>[2x]SNAMWKRMTA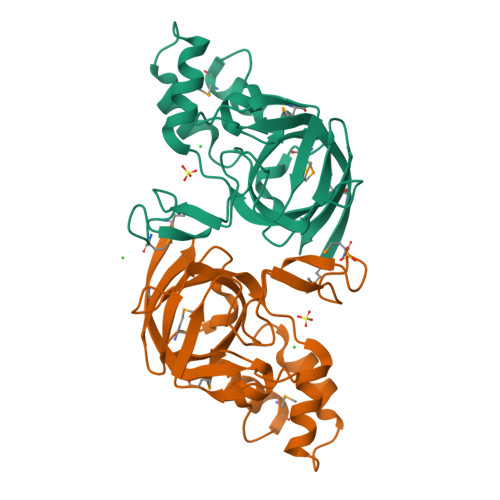KAEGLYIADTKSFVTKQMDKLDFDYGGIPGDLHFGLTKKAGAREPMFSRGTEIFNRRQISIVSIEECNEIALKMGVPRILPEWLGANVAVSGMPDLTSLKEGSRIIFPSGAALLCEGENDPCIQPGEVIQSYYPDQPKLASAFVRHALGIRGIVCIVERPGAVYTGDEIEVHSYQRKVKRKAERV[(2R,3S,4R,5R)-5-(6-amino-9H-purin-9-yl)-3,4-dihydroxytetrahydrofuran-2-yl]methyl 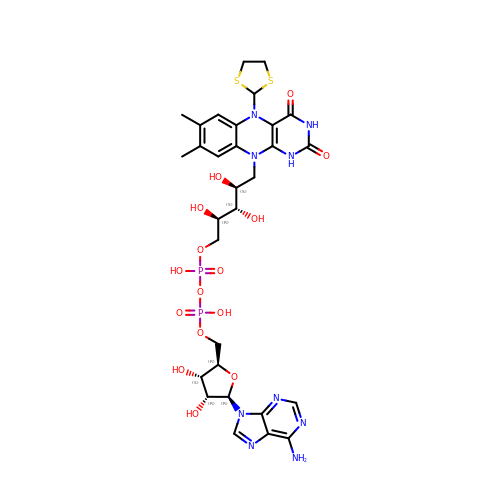(2R,3S,4S)-5-[5-(1,3-dithiolan-2-yl)-7,8-dimethyl-2,4-dioxo-1,3,4,5-tetrahydrobenzo[g]pteridin-10(2H)-yl]-2,3,4-trihydroxypentyl dihydrogen diphosphate | C30 H39 N9 O15 P2 S2 | JJIDBJDGDVTJIQ-LKQKGXMZSA-N>IVNSKRSELDKKISIAAKEIKSANAAEITPSRSSNEELEKELNRYAKAVGSLETAYKPFLASSALVPTTPTAFQNELKTFRDSLISSCKKKNILITDTSSWLGFQVYSTQAPSVQAASTLGFELKAIN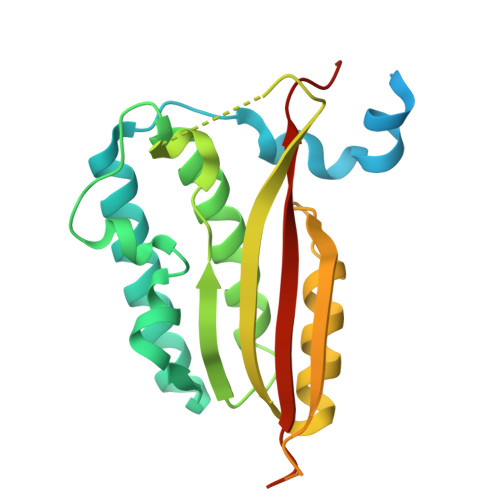SLVNKLAECGLSKFIKVYRPQLPIETPANNPEESDEADQAPWTPMPLEIAFQGDRESVLKAMNAITGMQDYLFTVNSIRIRNERMMPPPIANPAAAKPAAAQPATGAASLTPADEAAAPAAPAIQQVIKPYMGKEQVFVQVSLNLVHFNQPKAQEPSED[2x]> MKKVGNHNSISRKLLLSLSLTLIFSLTSFAQDPAAAPAATEAAAPAAASGGDPVKGKELFNANCAACHKLDAKSTGPALRGVASKHDMAWIYKWVHNSSDMIKSGDPVAVKLFEENNKAVMTSFPQLSTGDIDNIIAYTSEVKAEPAAAAGGAATPPGTNVEGGGISNNIILGALALVMAILVVMLFMVNKVLTKVASNNGIEVAPKEGRTPIWKAFAKNQFLVLVTSIFLLLASGYFVYGYLMQVGVDQNYEPIQPIHYSHKIHAGDNEINCKYCHSAARVSKTAGIPSLNVCMNCHKNISEVAETTATAEYSKAFYDAQIQKLYDAVGWDKTKQAYTGKTQPVKWVRIHNLPDFVYFNHSQHVSVAGVECQTCHGPVQEFEIMKQYSKLTMGWCVDCHRKTDVKMEGNAYYEKIHAELSKKYGVEKLTAAQMGGLECGKCHY;> CEGPVHKSIPYVLQPEQIIPGVADYYATTVFDGFDFANLLVKTREGRPIKIENNTIAGAKFSANARIHASILGLYDSMRLKEPKLDGKNSSWSAVDLKIKSSLADAKAKGGQVVLLTNTLASPTTEKLIGEFIAKNPNAKHVVYDAVSSSDALDAFETVYGERALVDYDFSKASLIVSVGADFLGDWQGGGYDAGYAKGRIPQNGKMSRHFQFESNMTLSGAAADKRVPMTTADQKQALVQIYNIVVGASVPVSLDAKFKAEVVKAAQQLKAAGTKGILVSGIEDKNAQLLVLAINQALASEAFSTAGTRQIRKGSNAVVAQLIKDMNAGSVHTLIMSGVNPVYTLADSASFVSGLKKVKTSVAFSLKEDETAAVSTIAAAAPHYLESWGDVEITKGTYSLTQPTIRPIFDTKQFQDVLLSVNGTPGNFYDYLKANSGAIIAGSSWNKVLHDGIFVVGSAALAGGSYDFAGAASLLSKAKSSGELELVLYTKTGMGDGQHANNPWLQEFPDPITRVSWDNYVTVSNADAKKFNLSNEIVANGGLNGSYATITTADGNKLENVPVIVQPGQAVGTVGLAVGYGRKAALKEEMQVGINAYALYKNFNSVQSITLAKANGEHEFACVQGQKTLMGRGDIIKETTLEIFNTQDAKHWNEQPMVSLDHQEVEATTVDLWESFDRTTGHHFNLSIDLNACTGCGACVIACHAENNVPVVGKAEVRRSRDMHWLRIDRYYSSESTFEGDNERKEGIAGLSSSLSTFNEMEKPGDNPQVAFQPVMCQHCNHAPCETVCPVAATSHGRQGQNHMAYNRCVGTRYCANNCPYKVRRFNWFLYNKNSEFDYHMNDDLGRMVLNPDVNVRSRGVMEKCSFCIQSTQAVILEAKRQGRVVGKDEFNNACACSAACSSGAMVFGDVNDKESEVAKLAESERMYHLLEHVGTKPNVFYHVKVRN;> MSSHYEAPIRKPLVIGDKSYHDVTVDVAAPVEGPANKQWWIVFTIALVAFLWGLGCIIYTVSTGIGTWGLNKTVGWAWDITNFVWWVGIGHAGTLISAVLLLFRQRWRMAINRSAEAMTIFSVVQAGLFPIIHMGRPWLAYWVLPIPNQFGSLWVNFNSPLLWDVFAISTYLSVSLVFWWTGLLPDFAMLRDRAITPFNKRVYSILSFGWSGRAKDWQRFEEVSLVLAGLATPLVLSVHTIVSMDFATSVIPGWHTTIFPPYFVAGAVFSGFAMVNTLLIVM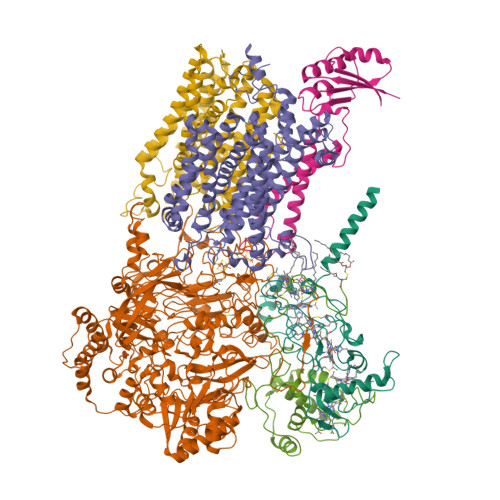RKVSNLEAYITLQHIELMNIIIMITGSIVGVAYITELFVAWYSGVEYEQYAFLNRATGPYWWAYWSMMTCNVFSPQFMWFKKLRTSIMFSFIISIVVNIGMWFERFVIIVTSLHRDYLPSSWTMFSPTFVDIGIFIGTIGFFFVLFLLYSRTFPVIAQAEVKTILKGTGDNYIRERANKDSHHE;> MSNKVIYAIYNDDDVLMNAVKKTRAAHHHIEEVFTPFPVHGLDKAMGLAPTRLAICAFLYGCVGISVATTMMSYIMIHDWPQDIGGKPSFSFIQNMPSFVPIMFEMTVFFAAHLMVITFYMRSRLWPFKQAENPDVRTTDDHFLIEVAVNDNEAELVSFFEGTGAVEVKVIEKN;> CHNNSAPNYQYFPNMYESVAYEPYTEAKIFKGGKEGQLPVEGTINRGFEPYEYENSTAGYELAKANLKSPLTEEEKNSGKGKELFEIYCISCHGAAGNGKGKLVEREKFLGVPSYKDREITEGSIFHVETYGLNAMGSHANQLSAHERWLVADYVLKLKSQL;> MYTFSSKLKTFSIILMVLGLLGIGYGFLSAPKDIQEVEKILAADAHGAHGTAHGESAEASHKEAGHHEAAEASHEEHKGGEHAKVGAADEHTEHLNHVLHQLQNKPWSALYVACIFFLLLSMGVLAFYAIQQVAQAGWSPVLFRVMQGITAYLPAGSIIFFIILVLCGLHFNHIFVWLGEGVTDPKSPNYDAIIAGKSGYLNFPFWIVRAFIFLLGWNIYRHFSRKNCLAQDEANDDLYYKKNFKISAGFLVFFIVSESIMAWDWIMSFDPHWFSTLFAWYVFASFFVSGITSIALITIYLKSKGYLEYVNTSHIHDLAKFMFGISVFWTYLWFSQFMLIWYANIPEEVTYFVTRIQLYNLPFFGAVVMNFVFPLLILINTDFKRLNWVVVMAGIVILLGHYVDFFNMIMPGTVGDKWFIGVPEIASILFFLGLFIFVVFTALTKSPLLAKRNPFIEESKHFHY> IPST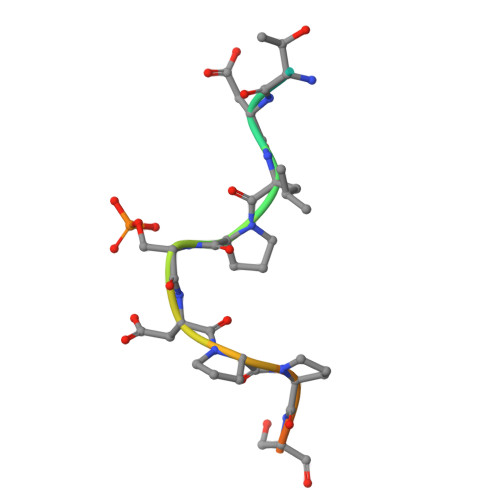DLPSDPPSDKEE>MIAQGQTLPNATLSQLTKEGMVHHPVLELFAGKKVVLFAVPGAFTPTCSEAHLPGYIVLADQLKAKGVDLIASVSVNDAFVMKAWGEAQNAEEILMLADGDASFTKALGLEMDTAGFGGLRSQRYAMIIDNGVVTTLNVEAPKSFEVSNAETILAALEHHHHHH[2x]

V. vulnificus Prx3 (VvPrx3) belongs to the 1-Cys class of Prxs, with one conserved catalytic cysteine (Cys48), and has been shown to be involved in pathogenicity in a mouse model. Cys48 is the CP residue that is crucial for the function of the protein. All three crystal structures of VvPrx3 revealed a protomer exhibiting a compact and spherical structure without a C-terminal extension region, similar to the previously reported 1-Cys Prx AhpE from Mycobacterium tuberculosis (Li et al., 2005). All three crystal structures of VvPrx3 [reduced Prx3 (C48D/C73S), oxidized Prx3 (C73S) and H2O2-bound Prx3 (C48D/C73S)] showed a similar dimeric assembly in the crystals characterized by an A-type dimeric interface, similar to that in AhpE from M. tuberculosis (Li et al., 2005).

To focus on the function of Cys48 and prevent unwanted disulfide-bond formation at Cys73 during SDS–PAGE analyses, Cys73 was replaced with a serine residue in this study. To investigate an oxidized structure of Prx3 containing a disulfide bond, the crystal of the oxidized VvPrx3 (C73S) protein was obtained under crystallization conditions without a reducing agent. The crystal structure of VvPrx3 (C73S) [named oxidized Prx (C73S) in this study] was determined at 1.5 Å resolution in space group P212121 using the molecular replacement method. Hydrophobic interactions were observed in the C-type interface that appear to further stabilize this dimeric interface. Owing to disulfide bonds and hydrophobic interactions, a significant conformational alteration was observed in the active site of helix α2 containing CP and nearby loops. The A-type dimer in the reduced state is further linked by the disulfide bond between the CP residues at the C-type interface, which can lead to the linear oligomer observed in oxidized Prx3 (C73S) crystals.Ribonucleotide reductases (RNRs) catalyze the conversion of ribonucleotides to deoxyribonucleotides, a conserved reaction that is fundamental to DNA-based life. Nearly all aerobic organisms use class I RNRs, which consist of two subunits: α, which contains the catalytic site, and β, which houses a subclass-dependent metal center. Contrary to all other class Ib RNRs studied to-date, the sole RNR of Bacillus subtilis displays class Ia-like activity regulation. We find that B. subtilis RNR has arrived at a remarkably similar solution to the ATP-cone through the evolution of two unique allosteric sites that modulate catalytic activity by inducing contrasting quaternary interactions that either enable or prevent the full range of motions needed for RNR activity.

A 6 Å resolution cryo-EM map was obtained of holo-NrdE under inhibiting conditions (100 µM dATP, 1 mM CDP), revealing an unusual double-helix with a hollow center. In this structure, each helical strand is composed of alternating I-dimer and S-dimer interfaces, leading to a non-terminating chain of NrdE subunits. Importantly, the simulated scattering from this double-helical model captures the distinct secondary scattering peak observed in the experimental scattering (black dashed), indicating that this structure is a stable species in solution. For both filaments, excess density at the S-site was modeled as dATP. As dATP acts as a specificity effector for CDP reduction, its presence at this site explains the formation of the S-dimer interface between adjacent I-dimer units. Additionally, a distinct, protruding density is observed at the I-site that is best explained as a dATP that displaced dAMP. In the NrdE-only filament, this cleft is unoccupied and partially buried by the double-helical interface formed by residues 660–665. Consistent with this, our cryo-EM maps of the dATP-induced filament display empty pockets at the M-site (purple stars).

>[4x]MSQNQVPKWIQLNNEIMIQKDGKFQFDKDKEAVHSYFVDYINQNTVFFHNLKEKLDYLVENQYYEEEFLSLYSFEDIKEVFKTAYAKKFRFPSFMSAFKFYNDYALKTNDKKKILERYEDRISIVALFFANGDTEKAKEYVNLMINQEYQPSTPTFLNAGRKRRGELVSCFLLEVNDSLNDISRAIDISMQLSKLGGGVSLNLSKLRAKGEAIKDVENATKGVVGVMKLLDNAFRYADQMGQRQGSGAAYLNIFHRDINDFLDTKKISADEDVRVKTLSIGVVIPDKFVELAREDKAAYVFYPHTIYKEYGQHMDEMDMNEMYDKFVDNPRVKKEKINPRKLLEKLAMLRSESGYPYIMFQDNVNKVHANNHISKVKFSNLCSEVLQASQVSSYTDYDEEDEIGLDISCNLGSLNILNVMEHKSIEKTVKLATDSLTHVSETTDIRNAPAVRRANKAMKSIGLGAMNLHGYLAQNGIAYESPEARDFANTFFMMVNFYSIQRSAEIAKEKGETFDQYEGSTYATGEYFDKYVSTDFSPKYEKIANLFEGMHIPTTEDWKKLKAFVAEHGMYHSYRLCIAPTGSISYVQSSTASVMPIMERIEERTYGNSKTYYPMPGLASNNWFFYKEAYDMDMFKVVDMIATIQQHIDQGISFTLFLKDTMTTRDLNRIDLYAHHRGIKTIYYARTKDTGQDSCLSCVV> PPPAIGQFWHVTDLHLDPTYHITDDHTKVCASSKGANASNPGPFGDVLCDSPYQLILSAFDFIKNSGQEASFMIWTGDSPPHVPVPELSTDTVINVITNMTTTIQSLFPNLQVFPALGNHDYWPQDQLPVVTSKVYNAVANLWKPWLDEEAISTLRKGGFYSQKVTTNPNLRIISLNTNLYYGPNIMTLNKTDPANQFEWLESTLNNSQQNKEKVYIIAHVPVGYLPSSQNITAMREYYNEKLIDIFQKYSDVIAGQFYGHTHRDSIMV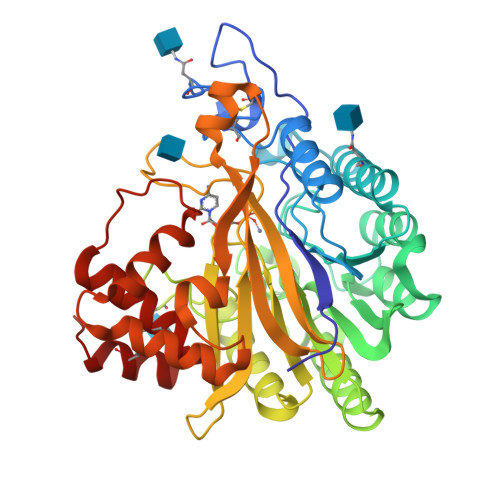LSDKKGSPVNSLFVAPAVTPVKSVLEKQTNNPGIRLFQYDPRDYKLLDMLQYYLNLTEANLKGESIWKLEYILTQTYDIEDLQPESLYGLAKQFTILDSKQFIKYYNYFFVSYDSSVTCDKTCKAFQICAIMNLDNISYADCLKQLYIK;>[2x]PPPAIGQFWHVTDLHLDPTYHITDDHTKVCASSKGANASNPGPFGDVLCDSPYQLILSAFDFIKNSGQEASFMIWTGDSPPHVPVPELSTDTVINVITNMTTTIQSLFPNLQVFPALGNHDYWPQDQLPVVTSKVYNAVANLWKPWLDEEAISTLRKGGFYSQKVTTNPNLRIISLNTNLYYGPNIMTLNKTDPANQFEWLESTLNNSQQNKEKVYIIAHVPVGYLPSSQNITAMREYYNEKLIDIFQKYSDVIAGQFYGHTHRDSIMVLSDKKGSPVNSLFVAPAVTPVKSVLEKQTNNPGIRLFQYDPRDYKLLDMLQYYLNLTEANLKGESIWKLEYILTQTYDIEDLQPESLYGLAKQFTILDSKQFIKYYNYFFVSYDSSVTCDKTCKAFQICAIMNLDNISYADCLKQL Recently, bioinformatics analyses have revealed the presence of CRISPR–Cas loci in bacterial Tn7-like transposons, thereby implicating a functional relationship between RNA-guided DNA targeting and transposition, with the latter representing a new role unrelated to host defense. Support for this concept has emerged from recent functional studies on type I-F and type V-K effectors involved in sequence-specific DNA transposition, thereby significantly broadening the potential biological applications of CRISPR–Cas technology. To complement the available functional studies, our efforts have focused on structural studies of the Vibrio cholerae Tn6677 multi-subunit type I-F CascadecrRNA–TniQ complex, whereby transposition subunit TniQ initiates DNA transposition with the eventual help of other transposition-associated proteins TnsA, TnsB and TnsC in the gene cluster. Here we report cryo-EM structures of a V. cholerae type I-F CascadecrRNA in complex with transposition subunit TniQ before (binary CascadecrRNA–TniQ) and after (ternary CascadecrRNA–TniQ–dsDNA) target double-stranded DNA (dsDNA) binding at an average resolution of 2.9 Å and 3.2 Å, respectively.

Cas6 and TniQ can be readily traced in the 2.9 Å structure of the binary complex, thereby providing insights into how the three Cas subunits (Cas8, Cas7, and Cas6) of the multi-subunit type I-F Cascade are assembled in an intertwined helical topology with crRNA and TniQ. The binary complex reveals a 1:6:1 Cas8:Cas7:Cas6 subunit stoichiometry similar to that reported for type I-F CascadecrRNA complexes, but contains a head-to-tail aligned TinQ dimer, whose individual monomers are bound to Cas7.1 and Cas6, so as to facilitate the first step of DNA transposition. The complex is assembled with a 60-nucleotide (nt) crRNA processed by the CRISPR-specific endoribonuclease Cas6 from long precursor CRISPR transcripts (pre-crRNA), which contains 28-nt repeat sequences separated by 32-nt plasmid- or phage-derived spacer sequences. Following Cas6-mediated maturation of crRNA, Cas proteins are assembled with crRNA, with the 5′ end recognized by Cas8 and the 3′ stem-loop held by Cas6, which is kinked by Cas7 thumb motifs in a periodic “5+1” pattern. Cas6 binds to the 3′ stem-loop of crRNA, while forming multiple polar interactions with Cas7.1 (left insert). Notably, the binary and DNA-bound ternary CascadecrRNA–TniQ complexes superpose with an RMSD of 2.33 Å. Minimal conformational changes are observed on ternary complex formation in the presence of bound target DNA, reflecting slight opening of the entire complex and crRNA, especially within the TniQ-bound end.

> MQTLKELIASNPDDLTTELKRAFRPLTPHIAIDGNELDALTILVNLTDKTDDQKDLLDRAKCKQKLRDEKWWASCINCVNYRQSHNPKFPDIRSEGVIRTQALGELPSFLLSSSKIPPYHWSYSHDSKYVNKSAFLTNEFCWDGEISCLGELLKDADHPLWNTLKKLGCSQKTCKAMAKQLADITLTTINVTLAPNYLTQISLPDSDTSYISLSPVASLSMQSHFHQRLQDENRHSAITRFSRTTNMGVTAMTCGGAFRMLKSGAKFSSPPHHRLNSKRSWLTSEHVQSLKQYQRLNKSLIPENSRIALRRKYKIELQNMVRSWFAMQDHTLDSNILIQHLNHDLSYLGATKRFAYDPAMTKLFTELLKRELSNSINNGEQHTNGSFLVLPNIRVCGATALSSPVTVGIPSLTAFFGFVHAFERNINRTTSSFRVESFAICVHQLHVEKRGLTAEFVEKGDGTISAPATRDDWQCDVVFSLILNTNFAQHIDQDTLVTSLPKRLARGSAKIAIDDFKHINSFSTLETAIESLPIEAGRWLSLYAQSNNNLSDLLAAMTEDHQLMASCVGYHLLEEPKDKPNSLRGYKHAIAECIIGLINSITFSSETDPNTIFWSLKNYQNYLVVQPRSINDETTDKSSL;>MKLPTNLAYERSIDPSDVCFFVVWPDDRKTPLTYNSRTLLGQMEAASLAYDVSGQPIKSATAEALAQGNPHQVDFCHVPYGASHIECSFSVSFSSELRQPYKCNSSKVKQTLVQLVELYETKIGWTELATRYLMNICNGKWLWKNTRKAYCWNIVLTPWPWNGEKVGFEDIRTNYTSRQDFKNNKNWSAIVEMIKTAFSSTDGLAIFEVRATLHLPTNAMVRPSQVFTEKESGSKSKSKTQNSRVFQSTTIDGERSPILGAFKTGAAIATIDDWYPEATEPLRVGRFGVHREDVTCYRHPSTGKDFFSILQQAEHYIEVLSANKTPAQETINDMHFLMANLIKGGMFQHKGD[6x];> MKWYYKTITFLPELCNNESLAAKCLRVLHGFNYQYETRNIGVSFPLWCDATVGKKISFVSKNKIELDLLLKQHYFVQMEQLQYFHISNTVLVPEDCTYVSFRRCQSIDKLTAAGLARKIRRLEKRALSRGEQFDPSSFAQKEHTAIAHYHSLGESSKQTNRNFRLNIRMLSEQPREGNSIFSSYGLSNSENSFQPVPLI;>MFLQRPKPYSDESLESFFIRVANKNGYGDVHRFLEATKRFLQDIDHNGYQTFPTDITRINPYSAKNSSSARTASFLKLAQLTFNEPPELLGLAINRTNMKYSPSTSAVVRGAEVFPRSLLRTHSIPCCPLCLRENGYASYLWHFQGYEYCHSHNVPLITTCSCGKEFDYRVSGLKGICCKCKEPITLTSRENGHEAACTVSNWLAGHESKPLPNLPKSYRWGLVHWWMGIKDSEFDHFSFVQFFSNWPRSFHSIIEDEVEFNLEHAVVSTSELRLKDLLGRLFFGSIRLPERNLQHNIILGELLCYLENRLWQDKGLIANLKMNALEATVMLNCSLDQIASMVEQRILKPNRKSKPNSPLDVTDYLFHFGDIFCLWLAEFQSDEFNRSFYVSRW[2x]>[2x]MSSILPFTPPIVKRLLGWKKGEQNGQEEKWCEKAVKSLVKKLKKTGQLDELEKAITTQNVNTKCITIPRSLDGRLQVSHRKGLPHVIYCRLWRWPDLHSHHELRAMELCEFAFN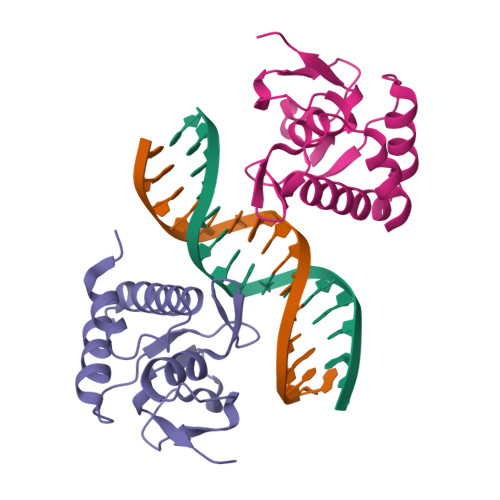MKKDEVCVNPYHYQRVETPVLPPVLVPRHT> GPHMGTSARDLLREMARDKPRLLAALEVASAAMAKEEAAGGEQDALDLYQHSLGELLLLLAAEPPGRRRELLHTEVQNL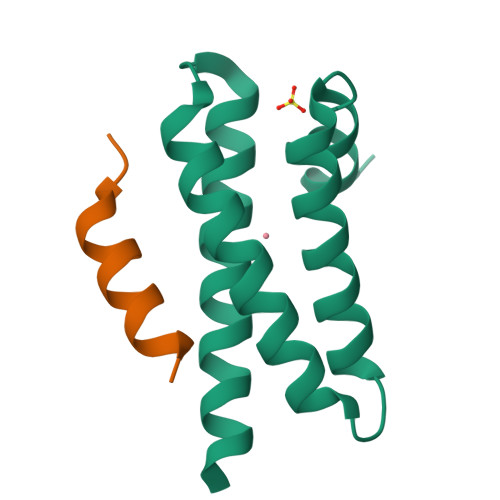MARAEYLKEQVKMRES;> TSASEDIDFDDLSRRFEELKKKT>STGLIKHTEYMEFLKSVPTFQSLPEEILSKLADVLEETHYENGEYIIRQGARGDTFFIISKGTVNVTREDSPSEDPVFLRTLGKGDWFGEKALQGEDVRTANVIAAEAVTCLVIDRDSFKHLIGGLDDVSNKAYEDAEAKAKYEAEAAFFANLKLSDFNIIDTLGVGGFGRVELVQLKSEESKTFAMKILKKRHIVDTRQQEHIRSEKQIMQGAHSDFIVRLYRTFKDSKYLYMLMEACLGGELWTILRDRGSFEDSTTRFYTACVVEAFAYLHSKGIIYRDLKPENLILDHRGYAKLVDFGFAKKIGFGKKTWTFCGTPEYVAPEIILNKGHDISADY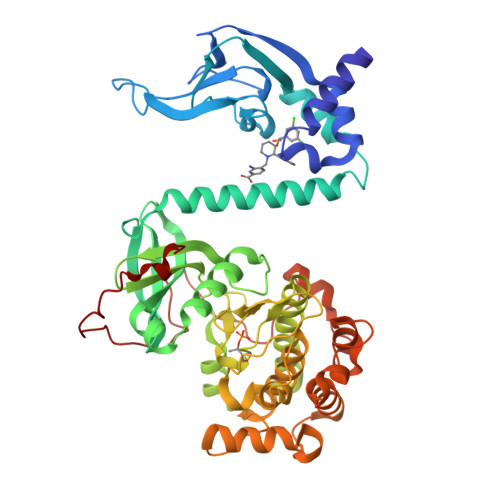WSLGILMYELLTGSPPFSGPDPMKTYNIILRGIDMIEFPKKIAKNAANLIKKLCRDNPSERLGNLKNGVKDIQKHKWFEGFNWEGLRKGTLTPPIIPSVASPTDTSNFDSFPEDNDEPPPDDNSGWDIDF[2x]>DGPGDGFTILSSKSLVLGQKLSLTQSDISHIGSMRVEGIVHPTTAEIDLKEDIGKALEKAGGKEFLETVKELRKS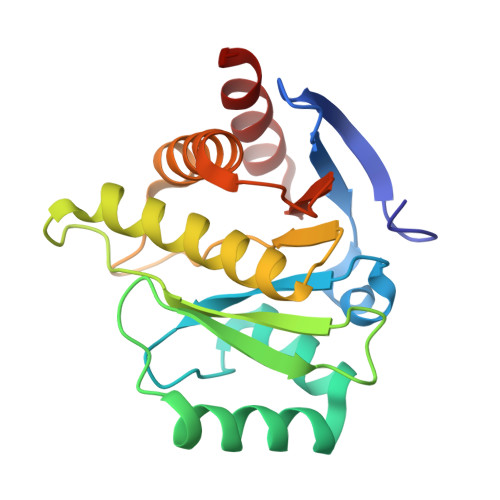QGPLEVAEAAVSQSSGLAAKFVIHCHIPQWGSDKCEEQLEETIKNCLSAAEDKKLKSVAFPPFPSGRNCFPKQTAAQVTLKAISAHFDDSSASSLKNVYFLLFDSESIGIYVQEMAKL[4x]> MHHHHHHHAVRASEISRVYEAYPEKKATLYFLVLGFLALIVGSLFGPFQALNYGNVDAYPLLKRLLPFVQSYYQGLTLHGVLNAIVFTQLFAQAIMVYLPARELNMRPNMGLMWLSWWMAFIGLVVFALPLLANEATVLYTFYPPLKGHWAFYLGASVFVLSTWVSIYIVLDLWRRWKAANPGKVTPLVTYMAVVFWLMWFLASLGLVLEAVLFLLPWSFGLVEGVDPLVARTLFWWTGHPILYFWLLPAYAIIYTILPKQAGGKLVSDPMARLAFLLFLLLSTPVGFHHQFADPGIDPTWKMIHSVLTLFVAVPSLMTAFTVAASLEFAGRL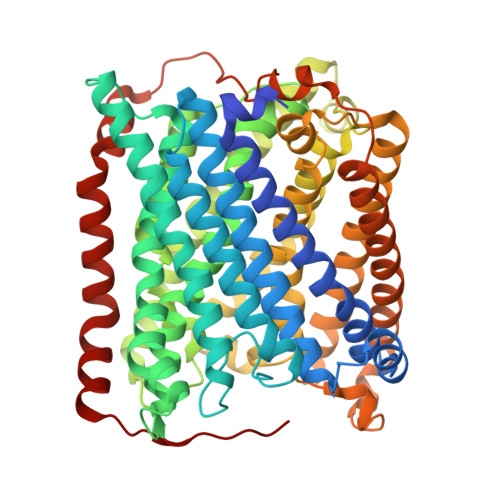RGGRGLFGWIRALPWDNPAFVAPVLGLLGFIPGGAGGIVNASFTLDYVVHNTAWVPGHFHLQVASLVTLTAMGSLYWLLPNLTGKPISDAQRRLGLAVVWLWFLGMMIMAVGLHWAGLLNVPRRAYIAQVPDAYPHAAVPMVFNVLAGIVLLVALLLFIYGLFSVLLSRERKPELAEAPLPFAEVISGPEDRRLVLAMDRIGFWFAVAAILVVLAYGPTLVQLFGHLNPVPGWRLW>GPHMLEQAHMGLSNGRPTGLNQIDSRAVAERINKYLEQLTAAATSATEEHFNELPRPHAVLDIIDALIQLIIKAQQTSEEFAIYALQQISQLLFRQPEGTLLLESLVHVLETIRKIAGPQVSEQVRQLFHQQPGHLFLSLSLIAALLGTDLLDWKNIDMAMAKALEQRKEGSIDFLEQLMDLV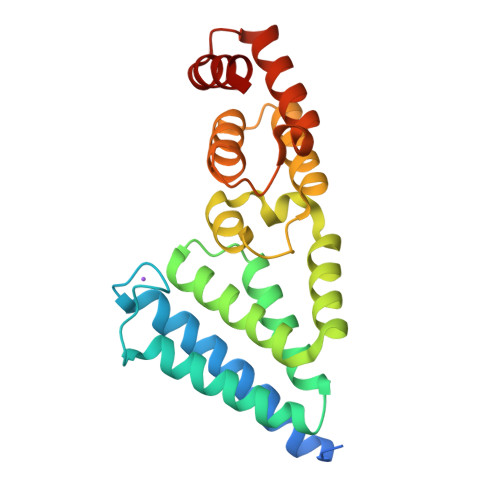LLNDTPLALFTDFVRSLEAAWAWIVEDPDLPAAQRFKAKVRAQ[2x]> MASLEDGTYRLRAVTTHNPDPGVGGEYATVEGARQPVKAEPSTPPFSEQQIWQVTRNSDGQYTIKYQGLNAPFEYGFSYDQLEPNAPVIAGDPKEYILQLVPSTADVYIIRAPIQRVGVDVEVGVQGNTLVYKFFPVDGSGGDRPAWRFTRE;> MASLEDGTYRLRAVTTHNPDPGVGGEYATVEGARQPVQAEPNTPPFFERQIWQVTRNADGQYTIKYQGLNAPFEYGFSYDQLEPNAPVIAGDPKEYILQLVPSTADVYIIRAPIQRVGVDVEVGVQGNTLVYKFFPVDGSGGDRPAWR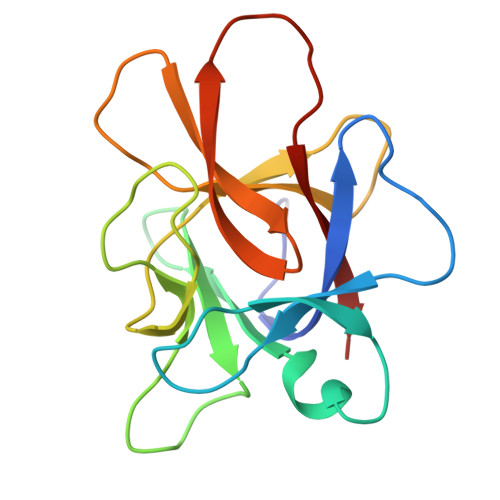FTRE>VRRDRAPPERGGAGTSQDGTSKNWFKITIPYGRKYDKAWLLSMIQSKCSVPFTPIEFHYENTRAQFFVEDASTASALKAVNYKILDRENRRISIIINSSAPPHTILNELKPEQVEQLKLIMSKRYDGSQQALDLKGLRSDPDLVAQNIDVVLNRRSCMAATLRII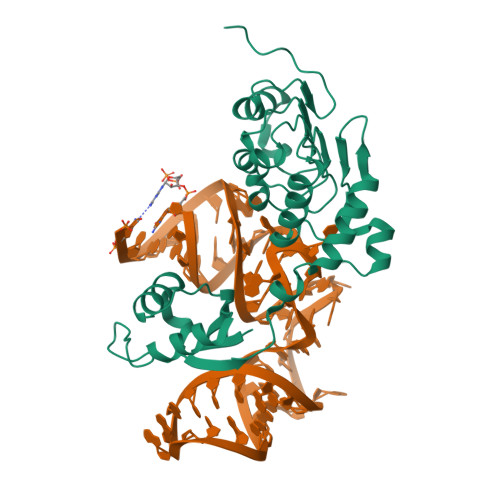EENIPELLSLNLSNNRLYRLDDMSSIVQKAPNLKILNLSGNELKSERELDKIKGLKLEELWLDGNSLCDTFRDQSTYISAIRERFPKLLRLDGHELPPPIAF[2x]>[2x]RSPWPPYKSSGIYEEEPQLPGASDLSGGVASDEIGVAPAQAVDERYRLPTTSIPIHYDLHLRTEIHRNERTFTGTVGIQLQVVQATDKLVMHNRGLVMSSAKVSSLPNGVTGAPTLIGDVQYSTDTTFEHITFTSPTILQPGTYLLEVAFQGRLATNDDGFYVSSYVADNGERRYLATTQFESTSARMAFPCYDEPGLKATFTVSITHSLSYKAISNMPQKTTTDIETDMRTTFFEKTPAMSTYLLAFVVSDFQLRLSGAQRVYVRPNAFNEATFALEAGVKILKVLDDHLGIPYDTYMPKLDQIAIPDFAAGAMENWGLVTYREQALLFNPAVSTYRGKTNVATTIAHEYAHQWFGNLVSPEWWEYIWLNEGFATLYEFYALDMAYPGQEYWELFNQQVIQYAMGQDGQASTRPMNWNAATPGEISALFDRVAYDKSGSVLNMMRHVLGDDNWKAGL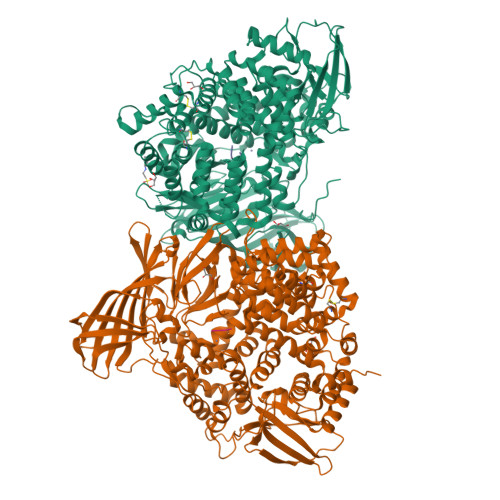KAYLTDRALQGAVDEQLYAGLQSAIEGKGVLPNGVTVAQIMRTWTNEAGYPVLNVRRSYDTGDVIISQERFYNDRKVPNTNIWMIPYNYVHQAKADFNEFDDFQWLATKAARIETTVPANEWIVFNKQQVGYYRVNYDEHNWELITNALHENWASIHRLNRAQLIDDAYWLARSGRLDLRVALRFMTYLRNEREYAPWTAANVALTYFNNRLRGTAEYHNFLIFVDALIEDIYSLLTIDAVSPDDTLLHKYLVQTISTWACSMGYTDCLMKTAALLKAEASGTGPAVHPDIASVTYCYGMRSALESEFQYLYRKMMNSKNLAERTMLIDSLGCSNNKEFLKAFLTTALGSGTGVEINYRADERRRVVQAIYSGGRTGVDALIEFLMDPALVNEFVSTLSTSTLNSALSAIASRTNNVEEMNKLNALITALGSRVNSQTAANLRTTAQANLDWVNGFEGLMLSNFLAEAAARGHPFEGKPIPNPLLGLDSTRTGHHHHHH;> AAAKA;> AAK>[2x]QNVSLQPPPQQLIVQNKTIDLPAVYQLNGGEEANPHAVKVLKELLSGKQSSKKGMLISIGEKGDKSVRKYSRQIPDHKEGYYLSVNEKEIVLAGNDERGTYYALQTFAQLLKDGKLPEVEIKDYPSVRYRGVVEGFYGTPWSHQARLSQLKFYGKNKMNTYIYGPKDDPYHSA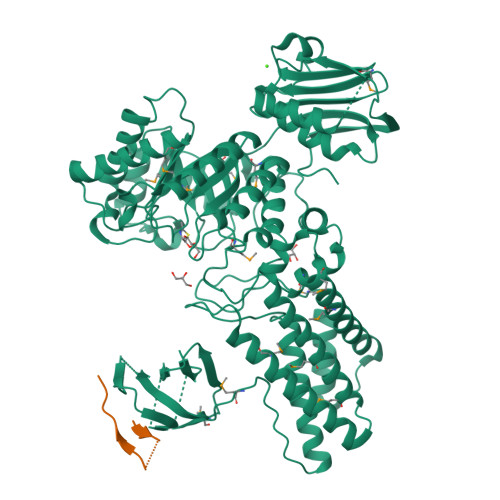PNWRLPYPDKEAAQLQELVAVANENEVDFVWAIHPGQDIKWNKEDRDLLLAKFEKMYQLGVRSFAVFFDDISGEGTNPQKQAELLNYIDEKFAQVKPDINQLVMCPTEYNKSWSNPNGNYLTTLGDKLNPSIQIMWTGDRVISDITRDGISWINERIKRPAYIWWNFPVSDYVRDHLLLGPVYGNDTTIAKEMSGFVTNPMEHAESSKIAIYSVASYAWNPAKYDTWQTWKDAIRTILPSAAEELECFAMHNSDLGPNGHGYRREESMDIQPAAERFLKAFKEGKNYDKADFETLQYTFERMKESADILLMNTENKPLIVEITPWVHQFKLTAEMGEEVLKMVEGRNESYFLRKYNHVKALQQQMFYIDQTSNQNPYQPGVKTATRVIKPLIDRTFATVVKFFNQKFNAHLDATTDYMPHKMISNVEQIKNLPLQVKANRVLISPANEVVKWAAGNSVEIELDAIYPGENIQINFGKDAPCTWGRLEISTDAKEWKTVDLKQKESRLSAGLQKAPVKFVRFTNVSDEEQQVYLRQFVLTIEKK>MLAKRIIACLDVKDGRVVKGTNFENLRDSGDPVELGKFYSEIGIDELVFLDITAFVEKRKTMLELVEKVAEQIDIPFTVGGGIHDFETASELILRGADKVSINTAAVENPSLITQIAQTFGSQAVVVAIDAKRVDGEFMVFTYSGKKNTGILLRDWVVEVEKRGAGEILLTSIDRDGTKSGYDTEMIRFVRPLTTLPIIASGGAGKMEHFLEAFLAGADAALAASVFHFREIDVRELKEYLKKHGVNVRLEGL[3x];>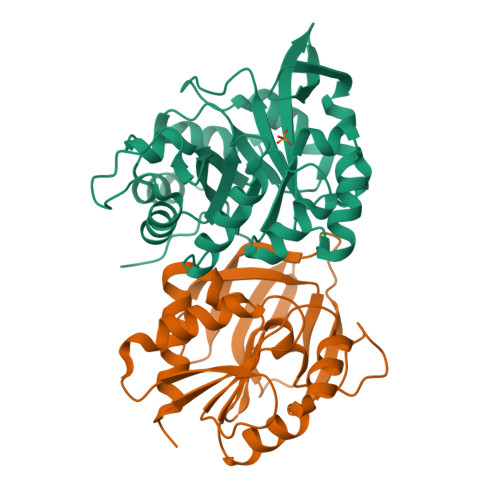MRIGIISVGPGNIMNLYRGVKRASENFEDVSIELVESPRNDLYDLLFIPGVGHFGEGMRRLRENDLIDFVRKHVEDERYVVGVCLGMQLLFEESEEAPGVKGLSLIEGNVVKLRSRRLPHMGWNEVIFKDTFPNGYYYFVHTYRAVCEEEHVLGTTEYDGEIFPSAVRKGRILGFQFHPEKSSKIGRKLLEKVIECSLSRR[3x]>[2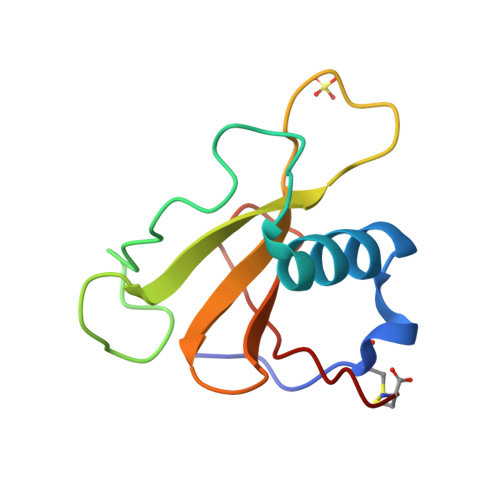x]DVSGTVCLSALPPEATDTLNLIASDGPFPYSQDGVVFQNRESVLPTQSYGYYHEYTVITPGARTRGTRRIICGEATQEDYYTGDHYATFSLIDQTC>RSPWCVICDPSVVLALKSLEKDYLPGHLDAKHHKAMMERVENAVKDFQELSLNEDAYMGVVDEATLQKGSWSLLKDLKRITDSDVKGDLFVKELFWMLHLQKETFATYVARFQKEAYCPNKCGVMLQTLIWCKNCKKEVHACRKSYDCGERNV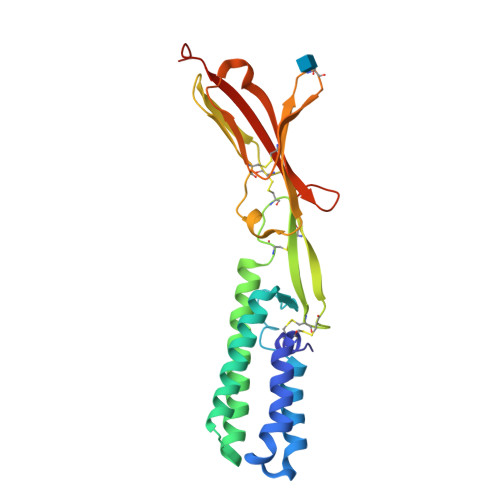EVPQMEDMILDCELNWHQASEGLTDYSFYRVWGNNTETLVSKGKEATLTKPMVGPEDAGSYRCELGSVNSSPATIINFHVTVLPKEFLEVLFQ[6x]>MTTSPTAPVALVTGAAKRLGSSIAEALHAEGYTVCLHYHRSAADASTLAATLNARRPNSA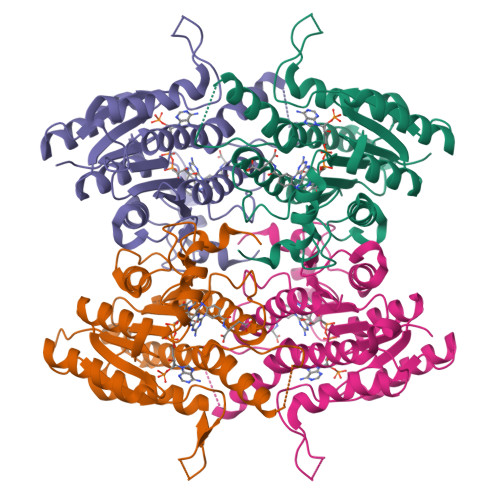ITVQADLSNVATASFSETDGSVPVTLFSRCSALVDACYMHWGRCDVLVNNASSFYPTPLLRKDAGEGGSSVGDKESLEVAAADLFGSNAIAPYFLIKAFAQRVADTRAEQRGTSYSIVNMVDAMTSQPLLGYTMYTMAKEALEGLTRSAALELASLQIRVNGVSPGLSVLPDDMPFSVQEDYRRKVPLYQRNSSAEEVSDVVIFLCSPKAKYITGTCIKVDGGYSLTRA[4x]>[2x]ASQTITVGSWGGPGGNGWDDGSYTGIRQIELSYKEAIGSFSVIYDLNGDPFSGPKHTSKLPYKNVKIELKFPDEFLESVSGYTGPFSALATPTPVVRSLTFKTNKGRTFGPYGDEEGTYF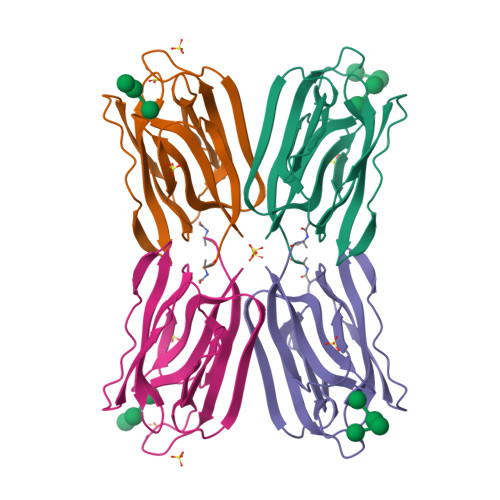NLPIENGLIVGFKGRTGDLLDAIGIHMSL> LTPDQQTLLHFIMDSYNKQRMPQEITNKILKEEFSAEENFLILTEMATNHVQVLVEFTKKLPGFQTLDHEDQIALLKGSAVEAMFLRSAEIFNKKLPSGHSDL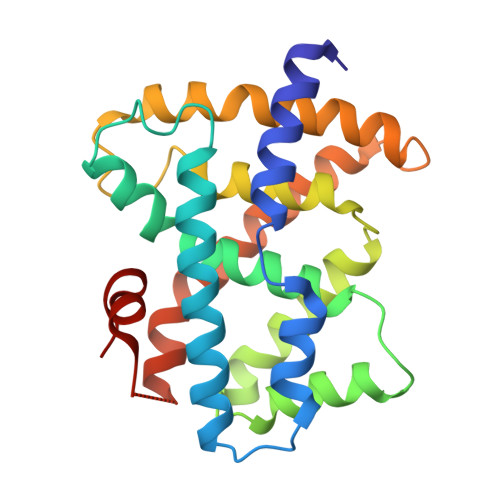LEERIRNSGISDEYITPMFSFYKSIGELKMTQEEYALLTAIVILSPDRQYIKDREAVEKLQEPLLDVLQKLCKIHQPENPQHFACLLGRLTELRTFNHHHAEMLMSWRVNDHKFTPLLCEIWDVQ>[2x]MHVVILGSA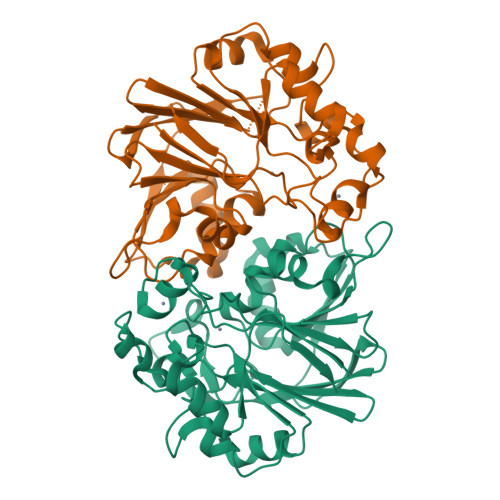AGGGVPQWNCRCSICSLAWAGDSRVRPRTQSSIAVSPDGERWLLLNASPDIRQQIQANPQMHPREGLRHSPIHAVLLTNGDVDHVAGLLTLREGQPFTLYATPGILASVSDNRVFDVMAADVVKRQTIALNETFEPVPGLSVTLFSVPGKVPLWLEDASMEIGAETETTVGTMIEAGGKRLAYIPGCARVTEDLKARIAGADALLFDGTVLEDDDMIRAGVGTKTGWRMGHIQMNGETGSIASLADIEIGRRVFVHINNTNPVLIEDSYERASVEARGWTVAHDGLTLDL> TIAPITGTIKRRVIMDIVLGFSLGGVMA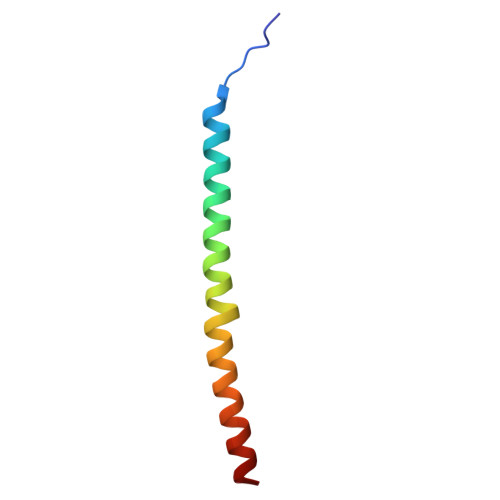SYWWWGFHMDKINKREKFYAELAERKK> SSHEQFRAALQLVVDPGDPRSYLDNFIKIGEGSTGIVCIATVRSSGKLVAVKKMDLRKQQRRELLFNEVVIMRDYQHENVVEMYNSYLVGDELWV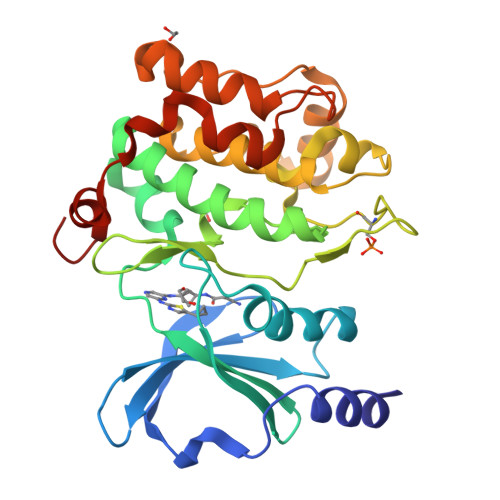VMEFLEGGALTDIVTHTRMNEEQIAAVCLAVLQALSVLHAQGVIHRDIKSDSILLTHDGRVKLSDFGFCAQVSKEVPRRKSLVGTPYWMAPELISRLPYGPEVDIWSLGIMVIEMVDGEPPYFNEPPLKAMKMIRDNLPPRLKNLHKVSPSLKGFLDRLLVRDPAQRATAAELLKHPFLAKAGPPASIVPLMRQNRTR> VEATAQETDRPRFSFSIAAREGKARTGTIEMKRGVIRTPAFMPVGTAATVKALKPETVRATGADIILGNTYHLMLRPGAERIAKLGGLHSFMGWDRPILTDSGGYQVMSLSSLTKQSEEGVTFKSHLDGSRHMLSPERSIEIQHLLGSDIVMAFDECTPYPATPSRAASSME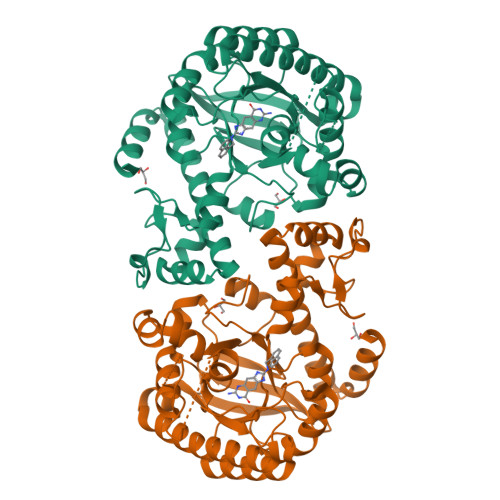RSMRWAKRSRDAFDSRKEQAENAALFGIQQGSVFENLRQQSADALAEIGFDGYAVGGLAVGEGQDEMFRVLDFSVPMLPDDKPHYLMGVGKPDDIVGAVERGIDMFDCVLPTRSGRNGQAFTWDGPINIRNARFSEDLKPLDSECHCAVCQKWSRAYIHHLIRAGEILGAMLMTEHNIAFYQQLMQKIRDSISEGRFSQFAQDFRARYFARNS> GPLGSPEFSSGNF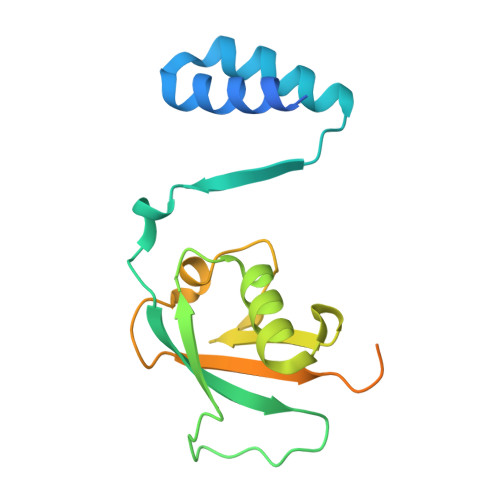KKEELATRLSQAIAGGDEKAAAQVAAVLAQHHVALNVQLMEAWFPPGPIRLQVTVEDATSVLSSSSSAHVSLKIHPHCSIAALQDQVFSEFGFPPAVQRWVIGRCLCMPERSLASYGVSQDGDPAFLYLLSAPREVSGQSLQNSKMDRKLGLFPQSLGLPHDLQPSSSSLPSPS> MTYKLYIMTFQNAHFGSGTLDSSKLTFSADRIFSALVLEA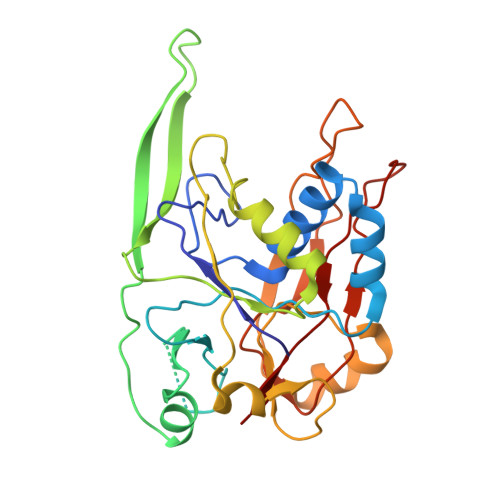LKMGKLDAFLAEANQDKFTLTDAFPFQFGPFLPKPIGYPKHDQIDQSVDVKEVRRQAKLSKKLQFLALENVDDYLNGELFENEEHAVIDTVTKNQPHKDDNLYQVATTRFSNDTSLYVIANESDLLNELMSSLQYSGLGGKRSSGFGRFELDIQNIPLELSDRLTKNHSDKVMSLTTALPVDADLEEAMEDGHYLLTKSSGFAFSHATNENYRKQDLYKFASGSTFSKTFEGQIVDVRPLDFPHAVLNYAKPLFFKLEV>[2x]MPATHHSSATSAERPTVVGRIPVLDVRPVVQRGRRPAKAVTGESFEVSATVFREGHDAVGANVVLRDPRGRPGPWTPMRELAPGTDRWGATVTAGETGTWSYTVEAWGDPVTTWRHHARIKIPAGLDTDLVLEEGARLYERAAADVPGREDRRELLAAVDALRDESRPAASRLAAALTPQVDAVLARHPLRDLVTSSDPLPLLVERERALYGAWYEFFPRSEGTPHTPHGTFRTAARRLPAIAAMGFDVVYLPPIHPIGTTHRKGRNNTLSATGDDVGSPWAIGSPEGGHDSIHPALGTLDDFDHFVTEAGKLGLEIALDFALQCSPDHPWVHKHPEWFHHRPDGTIAHAENPPKKYQDIYPIAFDADPDGLATETVRILRHWMDHGVRIFRVDNPHTKPVAFWERVIADINGTDPDVIFLAEAFTRPAMMATLAQIGFQQSYTYFTWRNTKQELTEYLTELSGEAASYMRPNFFANTPDILHAYLQ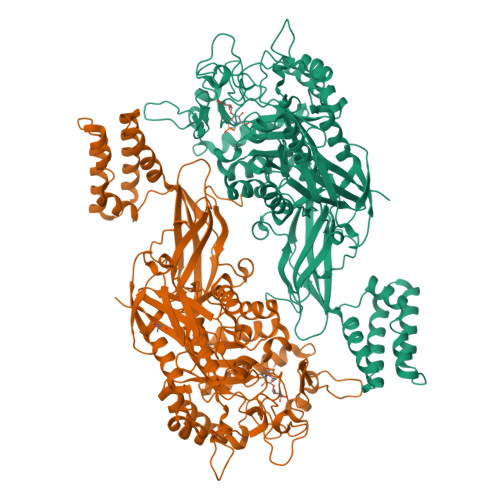HGGRPAFEVRAVLAATLSPTWGIYSGYELCENTPLREGSEEYLDSEKYQLKPRDWTRAAREGTTIAPLVTRLNTIRRENPALRQLRDLHFHPTDKEEVIAYSKRQGSNTVLVVVNLDPRHTQEATVSLDMPQLGLDWHESVPVRDELTGETYHWGRANYVRLEPGRTPAHVCTVLR>[4x]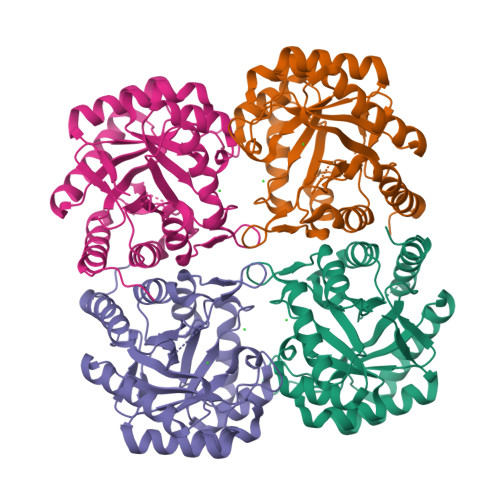MDIKINDITLGNNSPFVLFGGINVLESLDSTLQTCAHYVEVTRKLGIPYIFKASFDKANRSSIHSYRGVGLEEGLKIFEKVKAEFGIPVITDVHEPHQCQPVAEVCDVIQLPAFLARQTDLVVAMAKTGNVVNIKKPQFLSPSQMKNIVEKFHEAGNGKLILCERGSSFGYDNLVVDMLGFGVMKQTCGNLPVIFDVTHSLGRRAQALDLALAGMATRLAGLFLESHPDPKLAKCDGPSALPLHLLEDFLIRIKALDDLIKSQPILTIE>[2x]SPMAMTERLKVMTIFGTRPEAIKMAPLVLELQKHPEKIESIVTVTAQHRQMLDQVLSIFGITPDFDLNIMKDRQTL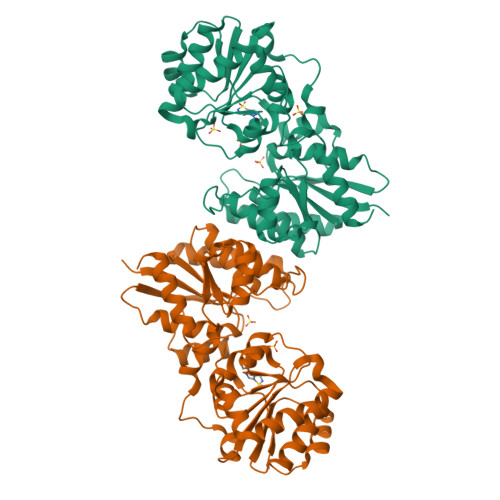IDITTRGLEGLDKVMKEAKPDIVLVHGDTTTTFIASLAAFYNQIPVGHVEAGLRTWDKYSPYPEEMNRQLTGVMADLHFSPTAKSATNLQKENKDESRIFITGNTAIDALKTTVKETYSHPVLEKLGNNRLVLMTAHRRENLGEPMRNMFRAIKRLVDKHEDVQVVYPVHMNPVVRETANDILGDYGRIHLIEPLDVIDFHNVAARSYLMLTDSGGVQEEAPSLGVPVLVLRDTTERPEGIEAGTLKLAGTDEETIFSLADELLSDKEAHDKMSKASNPYGDGRASERIVEAILKHFNK N-(4-quinazolin-4-ylphenyl)propanamide | C17 H15 N3 O | 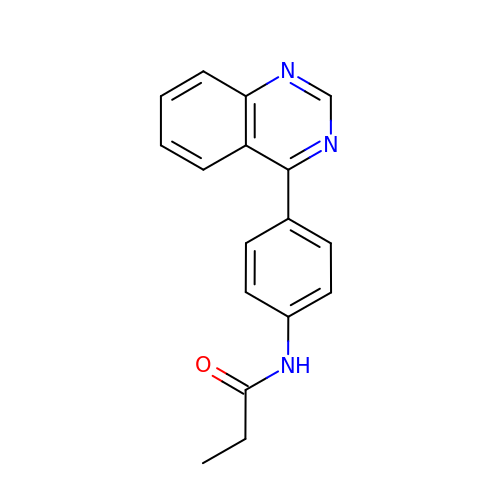MUOSBHKCWDCAKK-UHFFFAOYSA-N> MVSSFSVPMPVKRIFDTFPLQTYAAQTDKDEAVALEIQRRSYTFTERGGGSSELTVEGTYKLGVYNVFLEANTGAALATDPWCLFVQLALCQKNGLVLPTHSQEQTPSHTCNHEMLVLSRLSNPDEALPILVEGYKKRIIRSTVAISEIMRSRILDDAEQLMYYTLLDTVLYDCWITQIIFCASDAQFMELYSCQKLSGSIVTPLDVENSLLQKLSAKSLKISLTKRNKFQFRHREIV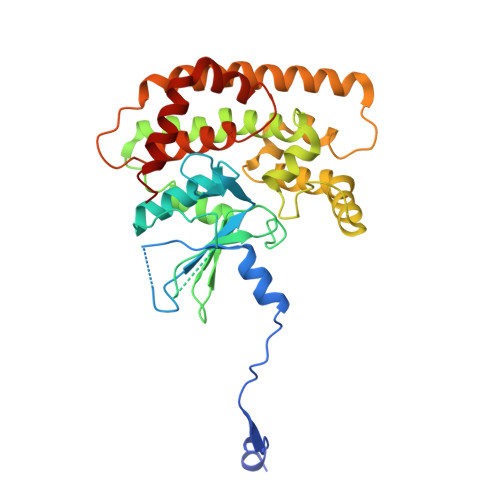KSMQGVYHNHHNSVNQEQVLNVLFENSKQVLLGLKDMLKSDGQPTYLHLKIASYILCITNVKEPIKLKTFVENECKELVQFAQDTLKNFVQ(3R)-4-[(4-CARBOXYBUTANOYL)OXY]-N-[(1E)-3-OXOPROP-1-EN-1-YL]-3-SULFINO-D-VALINE 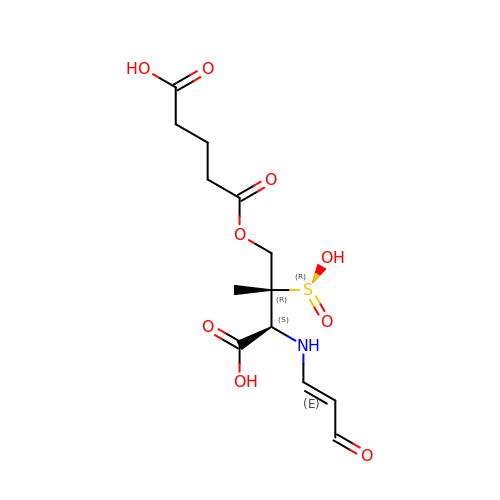| C13 H19 N O9 S | ZLJAMSCQNNEARN-QDZHIHTESA-N> ANITVFYNEDFQGKQVDLPPGNYTRAQLAALGIENNTISSVKVPPGVKAILYQNDGFAG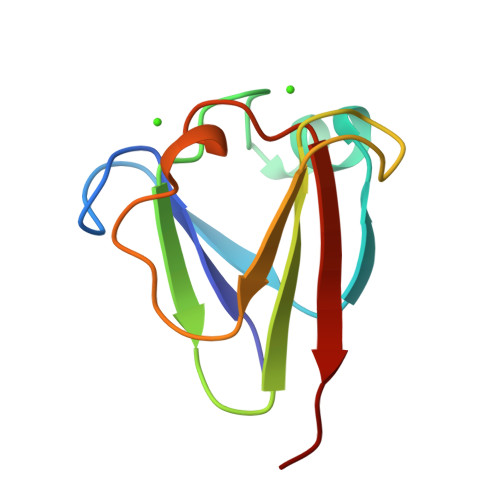DQIEVVANAEELGPLNNNVSSIRVISVPV> IVGGYTCAANSIPYQVSLNSGSHFCGGSLINSQWVVSAAHCYKSRI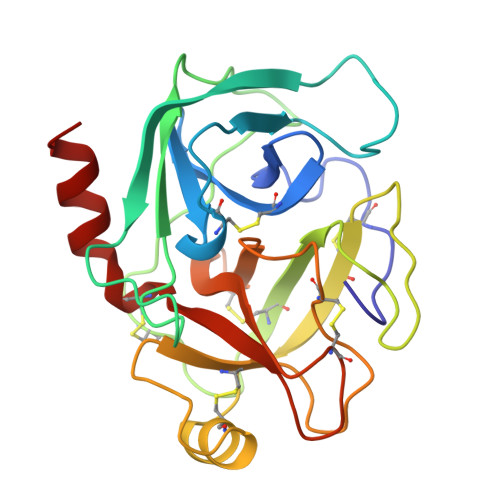QVRLGEHNIDVLEGNEQFINAAKIITHPNFNGNTLDNDIMLIKLSSPATLDSRVATVSLPRSCAAAGTECLISGWGNTKSSGSSYPSLLQCLKAPVLSDSSCKSSYPGQITGNMICVGFLEGGKDSCQGDSGGPVVCNGQLQGIVSWGYGCAQKNKPGVYTKVCNYVNWIQQTIAAN>CGCGGCAUUAAUGCAGCUUUAUUGCC[3x];>GGCAAUAAAGCGGUUACAAGCCCGCAAAAAUAGCAGAGUAAUGUCGCG[3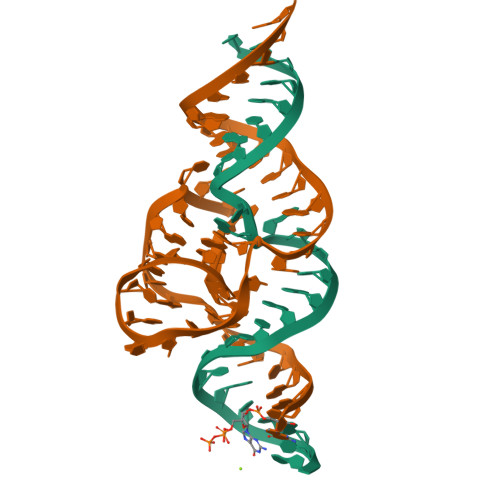x]>MHHHHHHHHHHGENLYFQGSSKHDYTNPPWNAKVPVQRAMQWMPISQKAGAAWGVDPQLITAIIAIQSGGNPNAVSKSNAIGLMQLKASTSGRDVYRRMGWSGEPTTSELKNPERNISMGAAYLNILETGPLAGIEDPK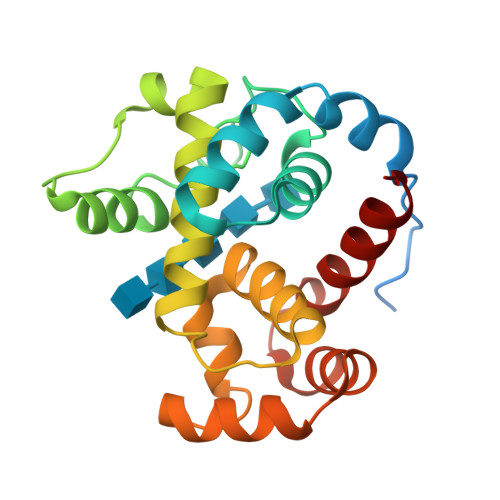VLQYALVVSYANGAGALLRTFSSDRKKAISKINDLDADEFLEHVARNHPAPQAPRYIYKLEQALDAM[2x]>MRGSHHHHHHGSNSNNICIDDNINTLWTGVNPTEANCQMMDSSESNDCKLILTLVKTGALVTAFVYVIGVSNNFNMLTTYRNINFTAELFFDSAGNLLTSLSSLKTPLNHKSGQNMATGAITNAKSFMPSTTAYPFNNNSRENYIYGTCHYTASDHTAFPI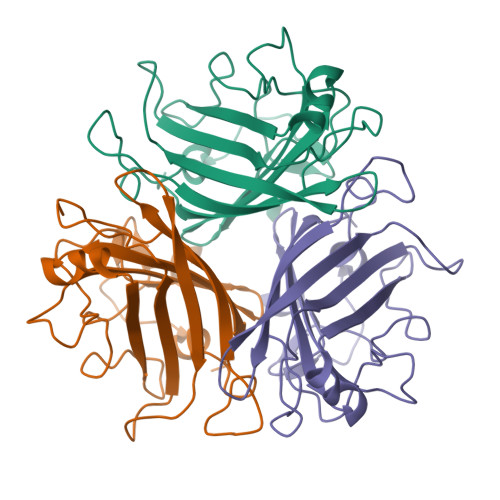DISVMLNQRAIRADTSYCIRITWSWNTGDAPEGQTSATTLVTSPFTFYYIREDD[3x]> MAMSNMTYNNVFDHAYEMLKENIRYDDIRDTDDLHDAIHMAADNAVPHYYADIFSVMASEGIDLEFEDSGLMPDTKDVIRILQARIYEQLTIDLWEDAEDLLN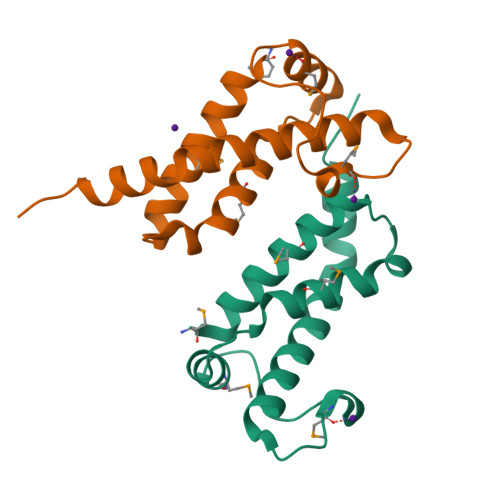EYLEEVEEYEEDEE benzyl [(1S)-2-(3-{[(4-carbamoylpiperidin-1-yl)(fluoro)oxo-lambda~6~-sulfanylidene]amino}phenyl)-1-cyanoethyl]carbamate | C23 H26 F N5 O4 S | 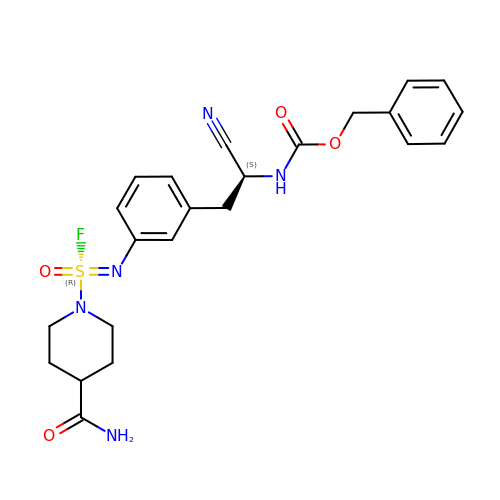HBDGRYHWGNZLEM-TXRXYBTHSA-N>[2x]MHRTSNGSHATGGNLPDVASHYPVAYEQTLDGTVGFVIDEMTPERATASVEVTDTLRERWGLVHGG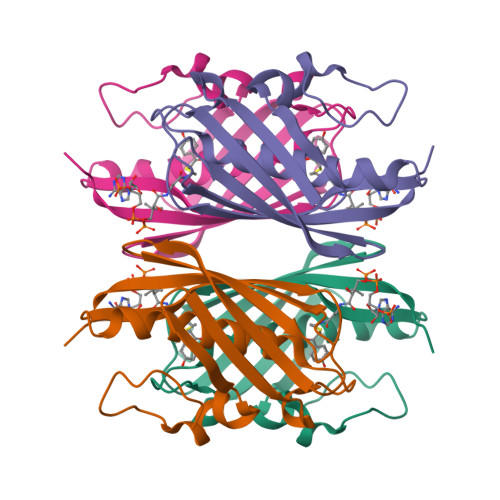AYCALAAMLATEATVAVVHEKGMMAVGQSNHTSFFRPVKEGHVRAEAVRIHAGSTTWFWDVSLRDDAGRLCAVSSMSIAVRPRRD>[2x]MTHVEVVATIAPQLYIEETLIQKINHRIDAIDVLELRIDQIENVTVNQVAEMITKLKVMQDSFKLLVTYRTKLQGGYGQF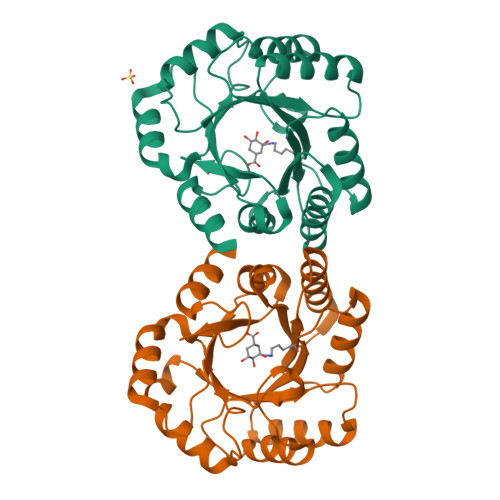TNDLYLNLISDLANINGIDMIDIEWQADIDIEKHQRIITHLQQYNKEVVISHHNFESTPPLDELQFIFFKMQKFNPEYVKLAVMPHNKNDVLNLLQAMSTFSDTMDCKVVGISMSKLGLISRTAQGVFGGALTYGCIGEPQAPGQIDVTDLKAQVTLY> GSHMLKKGMTTVLDFHPGAGKTRRFLPQILAECARRRLRTLVLAPTRVVLSEMKEAFHGLDVKFHTQAFSAHGSGREVIDAMCHATLTYRMLEPTRVVNWEVIIMDEAHFLDPASIAARGWAAHRARANESATILMTATPPGTSDEFPHSNGEIEDVQTDIPSEPWNTGHDWILADKRPTAWFLPSIRAANVMAASLRKAGKSVVVLNRKTFEREYPTIKQKKPDFILATDIAEMGANLCVERVLDCRTAFKPVLVDEGRKVAIKGPLRISASSAAQRRGRIGRNPNRDGDSYYYSEPTSENNAHHVCWLEASMLLDNMEVRGGM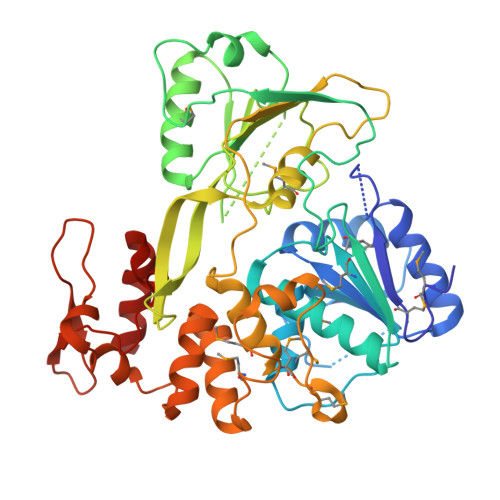VAPLYGVEGTKTPVSPGEMRLRDDQRKVFRELVRNCDLPVWLSWQVAKAGLKTNDRKWCFEGPEEHEILNDSGETVKCRAPGGAKKPLRPRWCDERVSSDQSALSEFIKFAEGRR> MPALKKQRIDLRLTDDDKSIIEEAAAISNQTITQFV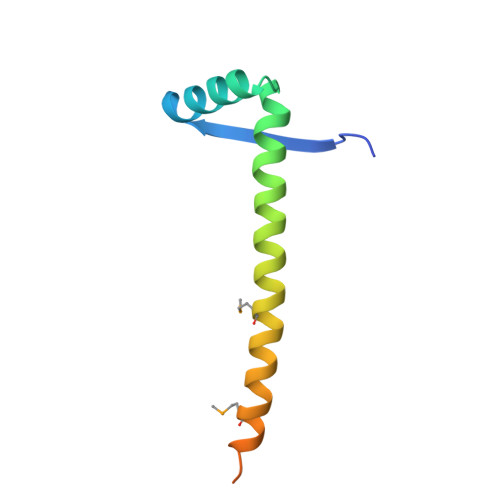VASASERAAEVIEQHRRMVLNEQSWSLVMEAITQPPAPNDRLKRAAKRLQTR> MDRPQE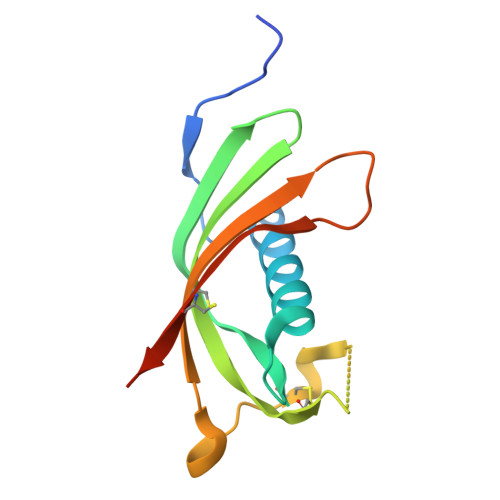RMVGELRDLSPDDPQVQKAAQAAVASYNMGSNSIYYFRDTHIIKAQSQLVAGIKYFLTMEMGSTDCRKTRVTGDHVDLTTCPLAAGAQQEKLRCDFEVLVVPWQNSSQLLKHNCVQMLEHHHHHH> MHELIKYQFNTRRKKYGTGAALSLLNGNVGHEVLAFHKKLPNYAVTPLHNLAHLSQRLGLGSIHIKDESWRFGLNAFKGLGGSYAVGKYLADKLQCDINSLSFAALNTPEI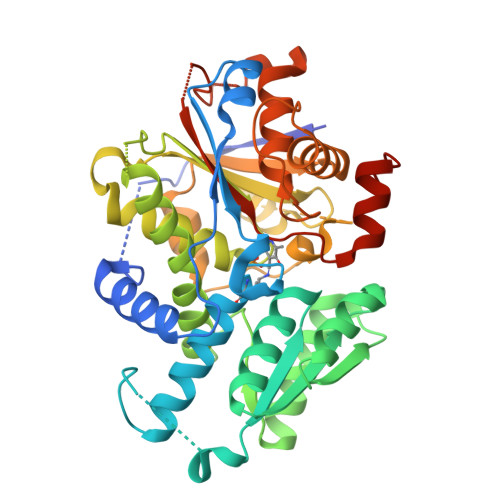KEKIKDCVFVTATDGNHGRGVAWAAEQLGLKAVVYMPKGSSLIRAENIRHHGAECTITDLNYDDAVRLAHRMAQTKGWVLLQDTAWTGYEEIPTWIMQGYMTLAVEAYEQLAETNSPLPTHLILQAGVGSFAGSVMGYFVEKMQENIPNIIVVEPHQANCLYQSAVMDDGQPHCVTGDMATIMAGLACGEPNIISWPIIRDNTSCFISADDCLAAKGMRISAAPRPGTDTPFISGESGAIGVGLLYELMNNMHYQDLANRLQLDASAHVLLISTEGDTSPDIYEDIVWNGRSALEHHHHHH>FSRRSHGDVKKSTQKVLDPKKDVLTRLKHLRALLDNVDANDLKQFFETNYSQIYFIFYENFIALENSLKLKGNNKSQREELDSILFLFEKILQFLPERIFFRWHYQSIGSTLKKLLHTGNSIKIRCEGIRLFLLWLQALQTNCAEEQVLIFACLVPGFPAVMSSRGPCTLETLINPSPSVADVKIYPEEITPLLPAISGEKIAEDQTCFFLQILLKYMVIQAASLEWKNKENQDTGFKFLFTLFRKYYLPHLFP[2x];>GPLGSGKGCKVVVCGLLSVGKTAILEQLLYGNHTIGMEDCETMEDVYMASVETDRGVKEQLHLYDTRGLQEGVELPKHYFSFADGFVLVYSVNNLESFQRVELLKKEIDKFKDKKEVAIVVLGNKIDLSEQRQVDAEVAQQWAKSEKVRLWEVTVTDRKTLIEPFTLLASKLSQPQSKS[2x]

κB-Ras1 and κB-Ras2 are small GTPases with noncanonical features that act as tumor suppressors downstream of Ras. Via interaction with the RalGAP (GTPase-activating protein) complex, they limit activity of Ral GTPases and restrict anchorage-independent proliferation. Other noncanonical GTPases of the Ras family are κB-Ras1 and κB-Ras2, which were originally identified as regulators of NF-κB signaling. In contrast to most GTPases, they lack a membrane targeting motif and a catalytic glutamine. κB-Ras GTPases not only show intrinsic GTP hydrolysis but also have fast nucleotide exchange rates, which shifts them into a constantly active form at physiological G-nucleotide concentrations.

We identified a fragment of RGα2 (RGα2N, residues 2–255) that forms a stable complex with κB-Ras1 (1–175) when coexpressed in bacterial cells. This RalGAP subcomplex was crystallizable, and we determined its structure at 2.72 Å resolution. κB-Ras1 adopts a canonical G domain fold comprised of a six-stranded central β-sheet and five α-helices. The N-terminal domain of RGα2 is composed of 10 helices forming tandem repeats that are twisted and have large loop insertions with short β-strand and α-helical elements. The nucleotide-binding pocket of κB-Ras1 is occupied by a magnesium ion and the nonhydrolyzable GTP analog 5′-guanylyl imidodiphosphate (GNP). Second, κB-Ras1 contains a leucine at position 65 instead of the catalytic glutamine 61, which is found at the equivalent position in Ras GTPases. Leu65 is tightly bound in a hydrophobic pocket formed by Cys10 of the β1-strand, Leu71 of switch II, and Leu100 of the α2-helix. The Gly64 carbonyl is oriented in a way that together with the backbone carbonyl of switch I Thr38, a water molecule could be coordinated in a position suitable for nucleophilic attack on the γ-phosphate of GTP. We observe no interactions of the κB-Ras1 switch region residues with RGα2N, consistent with previous findings that κB-Ras binding to RGα is nucleotide independent. The binding interface is constituted of helices α4 and α6 of RGα2N 10-helix bundle and the strands β1 and β2 of κB-Ras1 at the back side facing away from the nucleotide-binding pocket. Finally, a large loop inserted between α8 and α9 of RGα2 (V157–F211) folds back into a binding groove between α1 and β2 of κB-Ras1.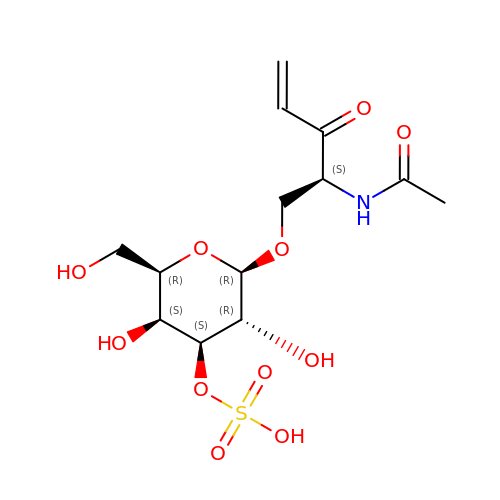[(2~{R},3~{R},4~{S},5~{S},6~{R})-2-[(2~{S})-2-acetamido-3-oxidanylidene-pent-4-enoxy]-6-(hydroxymethyl)-3,5-bis(oxidanyl)oxan-4-yl] hydrogen sulfate | C13 H21 N O11 S | XMURRHZYXOXPBZ-FJUAUIJYSA-N> GAMAPVTEKDLAEDAPWKKIQQNTFTRWCNEHLKCVNKRIGNLQTDLSDGLRLIALLEVLSQKRMYRKYHQRPTFRQMQLENVSVALEFLDRESIKLVSIDSKAIVDGNLKLILGLVWTL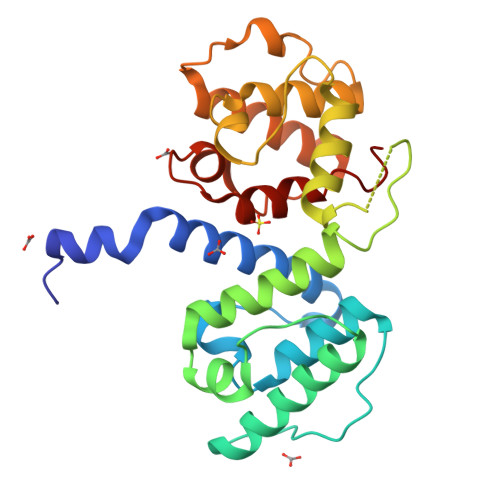ILHYSISMPVWEDEGDDDAKKQTPKQRLLGWIQNKIPYLPITNFNQNWQDGKALGALVDSCAPGLCPDWESWDPQKPVDNAREAMQQADDWLGVPQVITPEEIIHPDVDEHSVMTYLSQFPKAKL> GPGSMIKSTNIQAIGSGIMHQINNVYSLTPLSLPMELTPSMNEFYLKTWSEWEKNGTPGEQRNIAFNRLKICLQNQEAELNLSELDLKTLPDLPPQITTLEIRKNLLTHLPDLPPMLKVIHAQFNQLESLPALPETLEELNAGDNKIKELPFLPENLTHLRVHNNRLHILPLLPPELKLLVVSGNRLDSIPPFPDKLEGLALANNFIEQLPELPFSMNRAVLMNNNLTTLPESVLRLAQNAFVNVAGNPLSGHTMRTLQQITTGPDYSGPRIFFSMGNSATISAPEHSLADAVTAWFPENKQSDVSQIWHAFEHEEHANTFSAFLDRLSDTVSARNTSGFREQVAAWLEKLSASAELRQQSFAVAADATESCE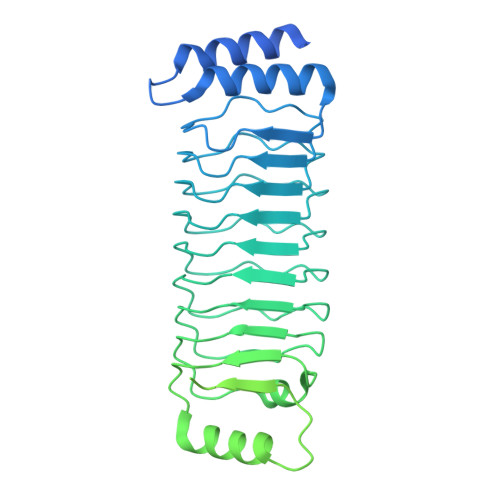DRVALTWNNLRKTLLVHQASEGLFDNDTGALLSLGREMFRLEILEDIARDKVRTLHFVDEIEVYLAFQTMLAEKLQLSTAVKEMRFYGVSGVTANDLRTAEAMVRSREENEFTDWFSLWGPWHAVLKRTEADRWAQAEEQKYEMLENEYSQRVADRLKASGLSGDADAEREAGAQVMRETEQQIYRQLTDEVLALRLSENGSNHIA> LSASPQPSSVAPRRPQE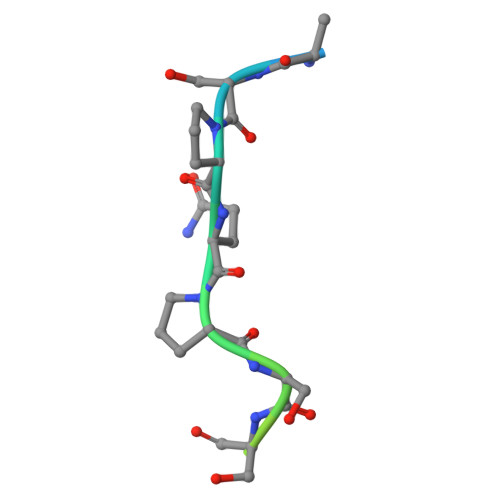PR> GPHMIKYTID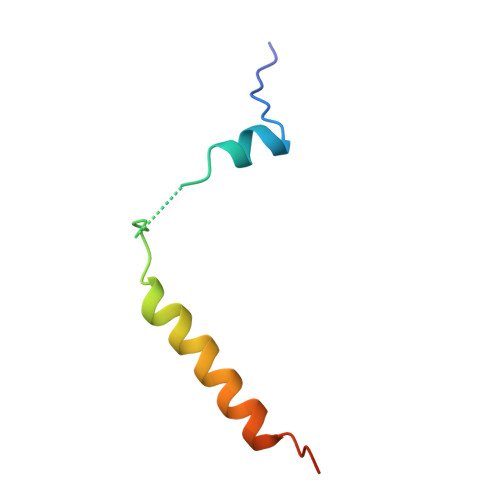ELFQLKPSLTLEVNFDAVEFRAIIEKVKQLQHLKEEEFNSHH> MIYMLGTNICVYAINKHPDSYYNNLELLAKN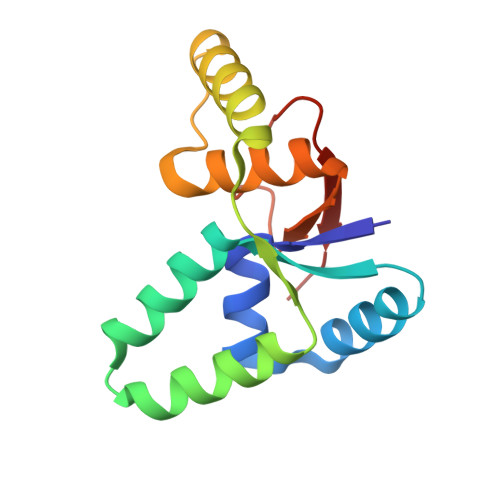NTIAISSIVLAELQYGVSKSKKKEQNQSKLDIFLSRLEIIDFSAKCTFYYGELRTELEQKGLIIGNNDLLIASHAIAENATLVTNNIKEFKRIPNLILENWDK> GPTGEAVERAIARVADTIGSGPVNSESIPALTAAETGHTSQVVPADTMQTRHVKNYHSRSESTVENFLCRSACVFYTTYRNHGTDGDNFGYWVISTRQVAQLRRKLEMFTYARFDLELTFVITSTQEQSTIQGQDSPVLTHQIMYVPPGGPVPTKVNSYSWQTSTNPSVFWTEGSAPPRMSIPFISIGNAYSMFYDGWAKFDKQGTYGINTLNNMGTLYMRHVNDGSPGPIVSTVRIYFKPKHVKTWVPRPPRLCQYQKAGNVNFEPTGVTESRTDITTMQTT;> SPSAEECGYSDRVRSITLGNSTITTQECANVVVGYGVWPTYLNDDEATAEDQPTQPDVATCRFYTLESVMWQQSSPGWWWKFPDALSNMGLFGQNMQYHYLGRAGYTVHVQCNASKFHQGCLLVVCVPEAEMGCATLANKPDQKSLSNGETANMFESQNSTGQTAVQANVINAGMGVGVGNLTIFPHQWINLRTNNSATIVMPYINSVPMDNMFRHNNFTLMIIPFAPLSYSTGATTYVPITVTVAPMCAEYNGLRLAGKQ;> GLPTMLTPGSNQFLTSDDFQSPSAMPQFDVTPEMDIPGQVNNLMEIAEVDSVVPVNNTEGKVLSIESYQIPVQSNSTNGSQVFGFPLMPGASSVLNRTLLGEILNYYTHWSGSIKLTFMFCGSAMATGKFLLA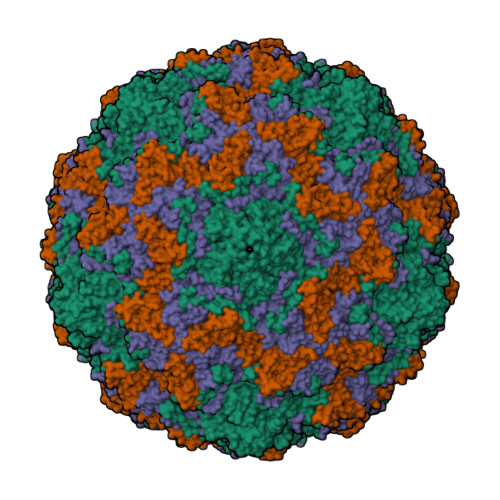YSPPGAGAPTTRKEAMLGTHVIWDVGLQSSCVLCIPWISQTHYRYVVVDEYTAGGYITCWYQTNIVVPADTQSDCKILCFVSACNDFSVRMLKDTPFIKQDNFYQ;> GAQVSTQKTGAHETGLSASGNSIIHYTNVNYYKDAASNSANRQDFTQDPGKFTEPVKDIMIKSMPALN>MAYVPLSGTNVRILADVPFSNDYKNTRWFTSSSNQYNWFNSKSRVYEMSKVTFMGFRENKPYVSVSLPIDKLYSASYIMFQNADYGNKWFYAFVTELEFKNSAVTYVHFEIDVLQTWMFDIKFQESFIVREHVKLWNDDGTPTINTIDEGLSYGSEYDIVSVENHKPYDDMMFLVIISKSIMHGTPGEEESRLNDINASLNGMPQPLCYYIHPFYKDGKVPKTYIGDNNANLSPIVNMLTNIFSQKSAVNDIVNMYVTDYIGLKLDYKNGDKELKLDKDMFEQAGIADDKHGNVDTIFVKKIPDYEALEIDTGDKWGGFTKDQESKLMMYPYCVTEITDFKGNHMNLKTEYINNSKLKIQVRGSLGVSNKVAYSVQDYNADSALSGGNRLTASLDSSLINNNPNDIAILNDYLSAYLQGNKNSLENQKSSILFNGIMGMIGGGISAGASAAGGSALGMASSV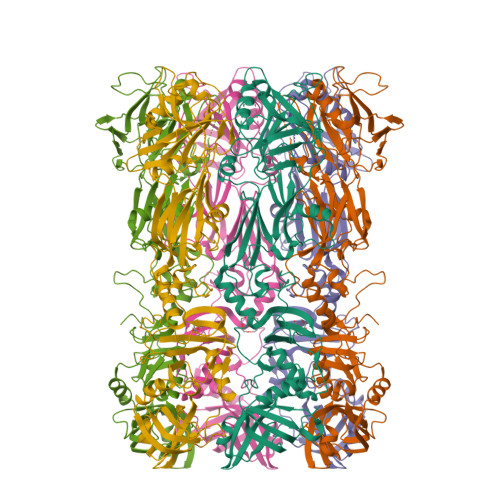TGMTSTAGNAVLQMQAMQAKQADIANIPPQLTKMGGNTAFDYGNGYRGVYVIKKQLKAEYRRSLSSFFHKYGYKINRVKKPNLRTRKAFNYVQTKDCFISGDINNNDLQEIRTIFDNGITLWHTDNIGNYSVENELRHHHHHH[3x]> VVGGEDAKPGQFPWQVVLNGKVDAFCGGSIVNEKWIVTAAHCVETGVKITVVAGEHNIEETEHTEQKRNVIRIIPHHNYNAAINKYNHDIALLELDEPLVLNSYVTPICIADKEYTNIFLKFGSGYVSGWGRVFHKGRSALVLQYLRVPLVDRATCLRSTKFTIYNNMFCAGFHEGGRDSCQGDAGGPHVT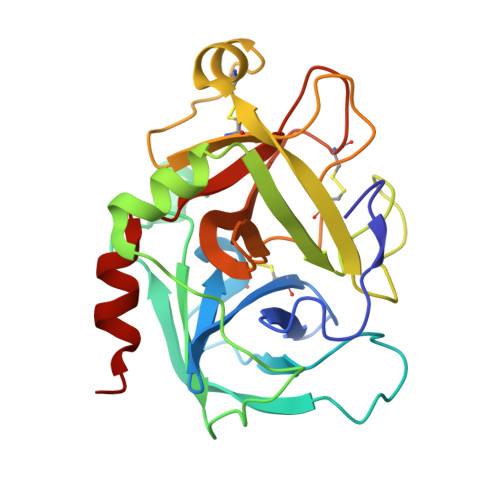EVEGTSFLTGIISWGEECAMKGKYGIYTKVSRYVNWIKEKTKLT> MQEPLAAGAVILRRFAFNAAEQLIRDINDVASQSPFRQMVTPGGYTMSVAMTNCGHLGWTTHRQGYLYSPIDPQTNKPWPAMPQSFHNLCQRAATAAGYPDFQPDACLINRYAPGAKLSLHQDKD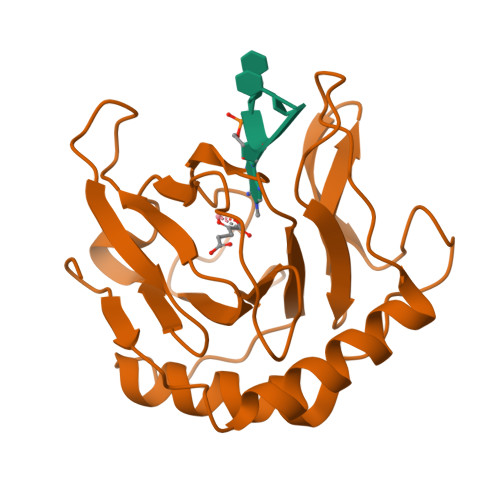EPDLRAPIVSVSLGLPAIFQFGGLKRNDPLKRLLLEHGDVVVWGGESRLFYHGIQPLKAGFHPLTIDCRYNLAFRQAGKKENLYFQ>MAKLLITGGCGFLGSNLASFALSQGIDLIVFDNLSRKGATDNLHWLSSLGNFEFVHGDIRNKNDVTRLITKYMPDSCFHLAGQVAMTTSIDNPCMDFEINVGGTLNLLEAVRQYNSNCNIIYSSTNKVYGDLEQYKYNETETRYTCVDKPNGYDESTQLDFHSPYGCSKGAADQYMLDYARIFGLNTVVFRHSSMY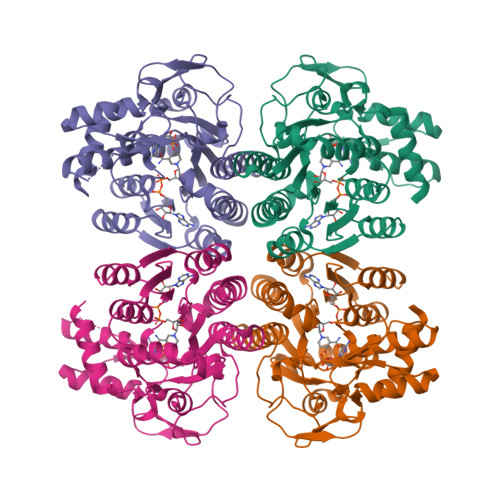GGRQFATYDQGWVGWFCQKAVEIKNGINKPFTISGNGKQVRDVLHAEDMISLYFTALANVSKIRGNAFNIGGTIVNSLSLLELFKLLEDYCNIDMRFTNLPVRESDQRVFVADIKKITNAIDWSPKVSAKDGVQKMYDWTSSILEHHHHHH[4x]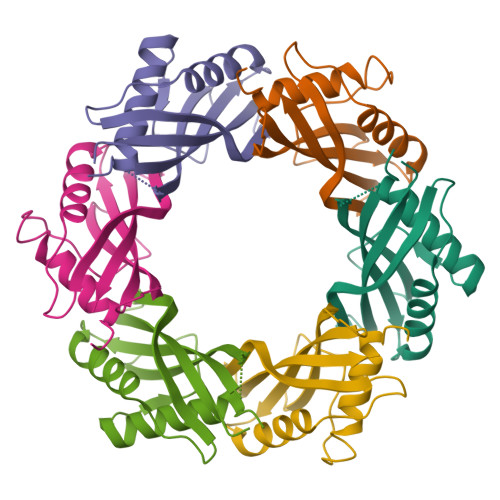> MKSLSFMRVLEAVRTMLQEKGGLDVSIVMRNQVEMPTTMIEMIDQEEEESQTAWKEKYRFAIHHYTNEQDLAGVEMIDTLIQMGFILPEGYKLVAVRHCGKQNLVKENTLIHAKTSFEVSICRELKVKI;> MKSLSFMRVLEAVRTMLEEKGGLDVSIVMRNQVEMPTTMIEMIDQEEEESQTAWKEKYRFAIHHYTNEQDLAGVEMIDTLIQMGFILPEGYKLVAVRHCGKQNLVKENTLIHAKTSFEVSICRELKVKI>CCTCTAGAGG[2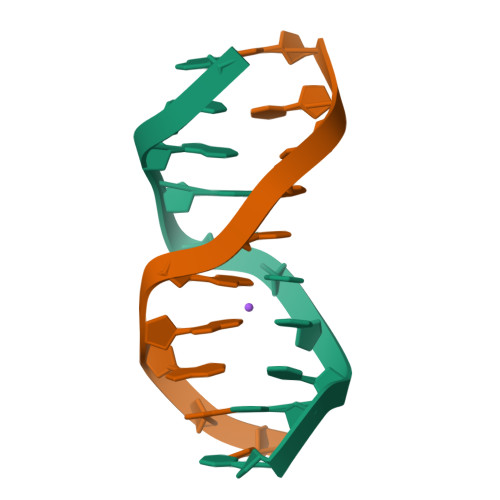x]>[4x]MFKPQPVTLRRGALCLEPLAEADLVEL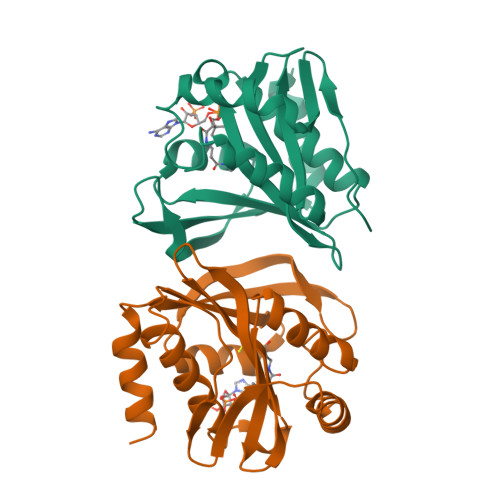LSLAEANRQSLIYMNGPLRPDWYRQGLAEQREGQAVIYAVRQDHALVGTTRFFDFMPGLPAVEIGGTWLAEDRHGSGLNAAIKFLMLRQAFEQWEMVRVQLKTAASNLRAQRAIEKLGARREGQLRNHRRLADGRLDDSILYSITDRDWPEIRRTLETELSAAARP> TNTRVNTLTPVTIKQILESKQDIQDGPFVSHNQELHHVCFVGVVRNITDHTANIFLTIEDGTGQIEVRKWSEDAA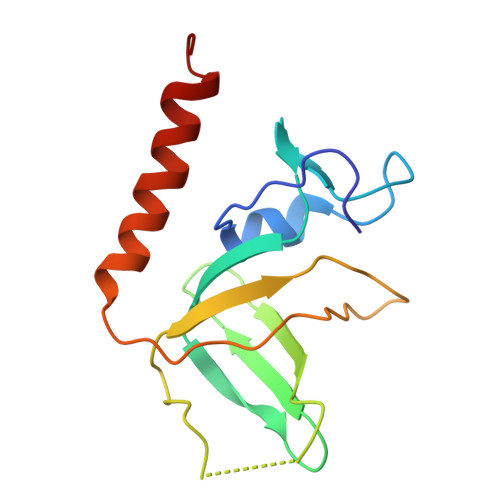QQFEIGGYVKVFGALKEFGGKKNIQYAVIKPIDSFNEVLTHHLEVIKCHSIASGMMK>GPLGSDLITCYCRKPFAGRPMIECSLCGTWIHLSCAKIKKTNVPDF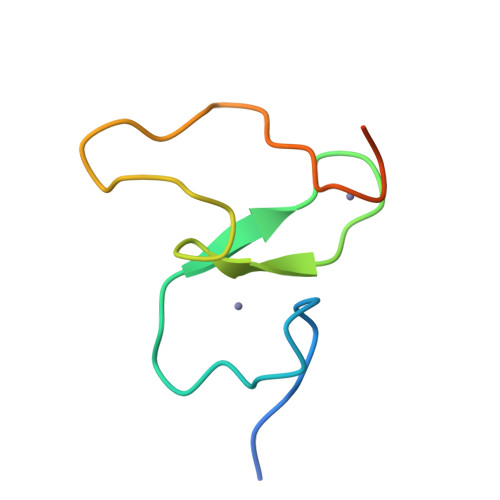FYCQKCKELRPEARR[5x]N-((1S,2R)-1-hydroxy-1-(o-tolyl)pentan-2-yl)-2-oxo-2,3-dihydrobenzo[d]oxazole-5-carboxamide | C20 H22 N2 O4 | 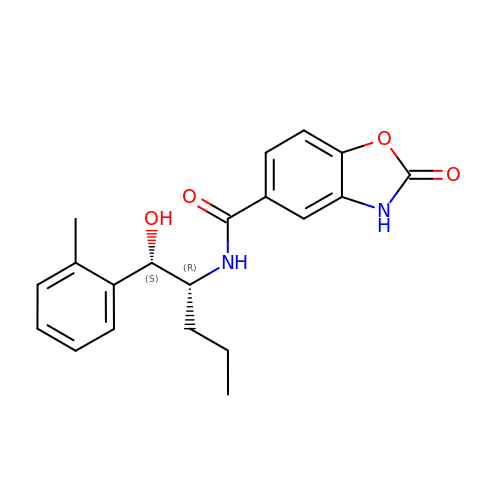SNFRXTGIONJORR-QAPCUYQASA-N>MGLEKTVKEKLSFEGVGIHTGEYSKLIIHPEKEGTGIRFFKNGVYIPARHEFVVHTNHSTDLGFKGQRIKTVEHILSVLHLLEITNVTIEVIGNEIPILDGSGWEFYEAIRKNILNQNREIDYFVVEEPIIVEDEGRLIKAEPSDTLEVTYEGEFKNFL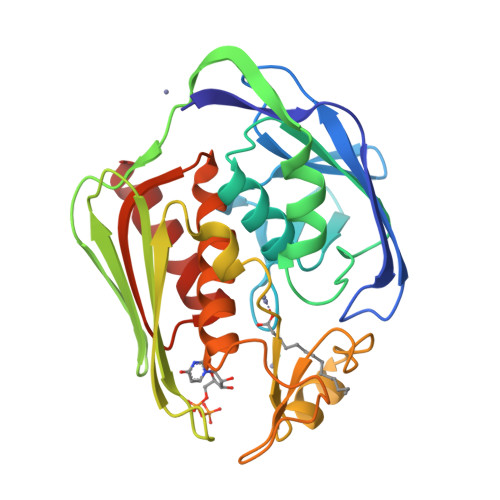GRQKFTFVEGNEEEIVLARTFAFDWEIEHIKKVGLGKGGSLKNTLVLGKDKVYNPEGLRYENEPVRHKVFDLIGDLYLLGSPVKGKFYSFRGGHSLNVKLVKELAKKQKLTR[2x]> MKKISRKEYVSMYGPTTGDKVRLGDTDLIAEVEHDYTIYGEELKFGGGKTLREGMSQSNNPSKEELDLIITNALIVDYTGIYKADIGIKDGKIAGIGKGGNKDMQDGVKNNLSVGPATEALAGEGLIVTAGGIDTHIHFISPQQIPTAFASGVTTMIGGGTGPADGTNATTITPGRRNLKWMLRAAEEYSMNLGFLAKGNASNDASLADQIEAGAIGFKIHED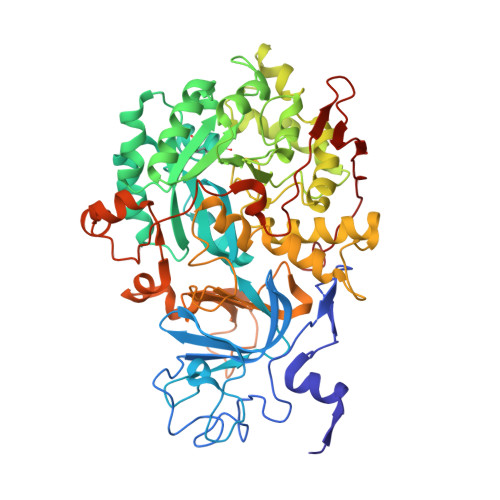WGTTPSAINHALDVADKYDVQVAIHTDTLNEAGCVEDTMAAIAGRTMHTFHTEGAGGGHAPDIIKVAGEHNILPASTNPTIPFTVNTEAEHMDMLMVCHHLDKSIKEDVQFADSRIRPQTIAAEDTLHDMGAFSITSSDSQAMGRVGEVITRTWQTADKNKKEFGRLKEEKGDNDNFRIKRYLSKYTINPAIAHGISEYVGSVEVGKVADLVLWSPAFFGVKPNMIIKGGFIALSQMGDANASIPTPQPVYYREMFAHHGKAKYDANITFVSQAAYDKGIKEELGLERQVLPVKNCRNVTKKDMQFNNTTAHIEVNPETYHVFVDGKEVTSKPANKVSLAQLFSIF OXALATE ION | C2 O4 | 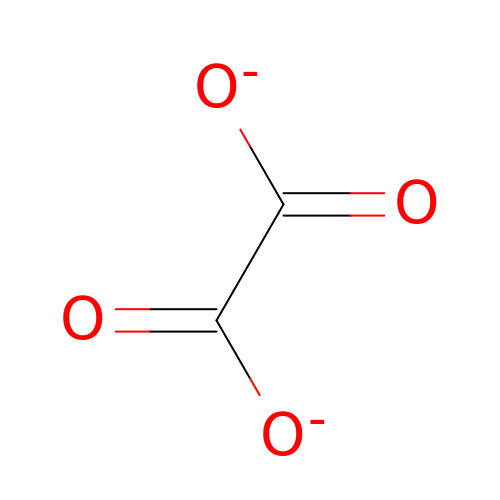MUBZPKHOEPUJKR-UHFFFAOYSA-L> SNKVGTLQAQVEATQKQKAQPIDANRKYDYKLQYYLNDYVYAYFTLPQEGDKQQAQVEHLNSFYNFVPDVKAQGQVRNPSTLLDSQLVTVEGKVATYKVKYKEMIQHDKDTEEKELVTGFNIPFDEKEGKYYVSGLPWFSA

In this study, we combined structural, biochemical and biophysical approaches to study OrfG, a protein that belongs to Conj-T4SS of ICESt3 from Streptococcus thermophilus. A structural analysis revealed that the OrfG central domain adopts a NTF2-like fold and likely presents more structural similarities with VirB8-like proteins TcpC and TraM from Gram-positive bacteria than Gram-negative VirB8 proteins. Consequently, we propose that OrfG operates as a VirB8-like protein in the conjugative apparatus of ICESt3. Biochemical and biophysical characterizations of purified OrfG soluble domain and its central and C-terminal subdomains indicated that they are mainly monomeric in solution but able to form an unprecedented 6-mer oligomers.

To overcome these technical issues, and based on the secondary structure prediction of OrfG as well as the sequence alignment between OrfG and TcpC, we chose to express and purify to homogeneity the separate central (OrfG64–204: from Ser64 to Ala204) and C-terminal (OrfG223–331: from Ala223 to Asp331) subdomains. Crystallization trials conducted on both forms resulted in suitable tetragonal crystals for OrfG64–204 while no positive result was obtained for OrfG223–331. Experimental phases were determined by using a single-wavelength anomalous dispersion method on crystals soaked with an osmium derivative. A native crystal allowed final model refinement to 1.75 Å resolution (R free = 20.8%). The polypeptide chain adopts an alpha + beta fold, composed of two α-helices named α 1 and α 2, followed by a β-sheet of four strands (β1–β4), the last of which has a marked disruption into two subparts β4a and β4b. Indeed, OrfG64–204 has no α 3 (replaced by an unobservable region) and a strand β4 that clearly splits in two short portions β4a and β4b separated by a bulge that ends with Pro200. Note that the electron density of OrfG central domain displayed a blob that remained unassigned despite attempts to fit various compounds in it. This density was located between β4 and the C-terminal end of α1. Surprisingly, the electron density of OrfG central domain displayed an unassigned blob nicely docked in a pocket localized in a hydrophobic cavity that shares intriguing similarity with the groove identified in Gram-negative VirB8 proteins. Thus, the localization of this groove suggests a probable oligomerization inhibition site for OrfG.>[2x]MSQFDLTPPSPAQRDALIAGLSDEEQRVLLH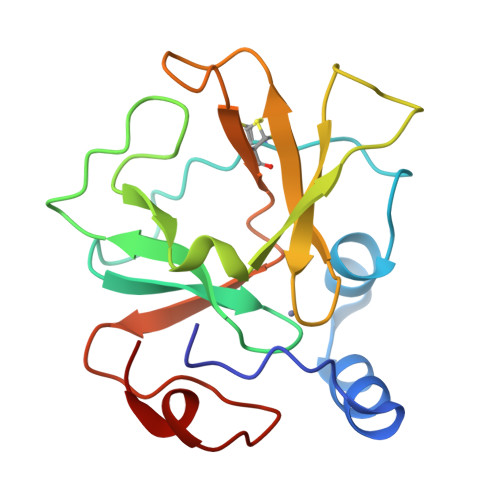HGTEAPFCGVFLDNKLDGVYTCRLCGLPLFRSNAKFDSGTGWPSFFAPYDPAHVREIRDTSYGMIRTEIVCARCDSHLGHVFPDGPPPTGERHCLNSVSLAFTEDGQPLPNPLQRAGAETQPA> MSGIAEFDGILDSLEHSKTGISGSKILKLTNLSMENVSENAQFVASVYKYAKRAPVTHKLGALYILDSIVRSFQDGAKKNNESFENPVDASFSGGWCKA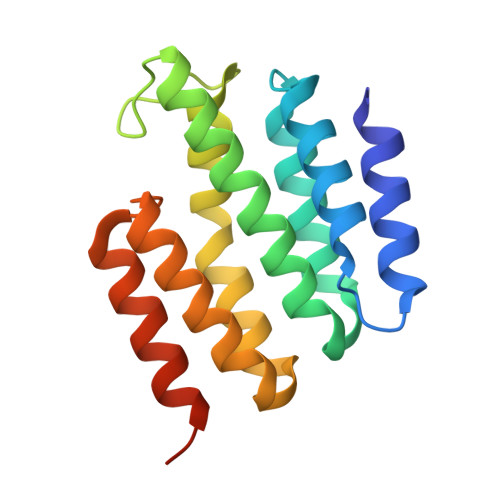AEITDSLVADAIQHAPSAHLPKILKLCDIWEKASTFPPEKLESLRSKLKDAMALEHHHHHHHH>[2x]MAHHHHHHM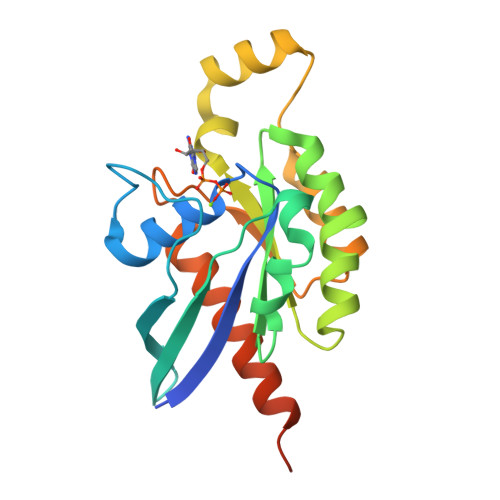ESIKCVVVGDGAVGKTALLIAYSSGCFPEDYVPTVFDNYNKNIPYGDGIVSIALYDTAGQEDYDRLRPLSYPDTDVFLVCFSLENPNSLENCHSKWAEELKHYNPDTPIVLVGTKLDLKKDEEYVKKLKEKKISPVTTEQGQEMKDKIKACGYIECSAKTMENLTEAFNMAIDIAMKQRLKDAPPTANARNQKKKCQLL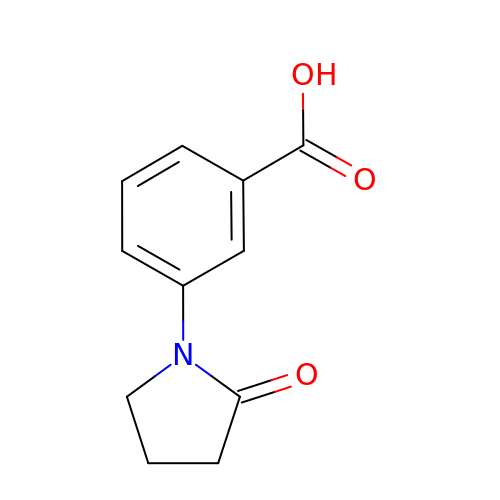3-(2-oxopyrrolidin-1-yl)benzoic acid | C11 H11 N O3 | QESXXFDZRITHKE-UHFFFAOYSA-N(2~{S})-4-[[(2~{S},3~{S},4~{R},5~{R})-5-(6-aminopurin-9-yl)-3-[[(2~{R},3~{S},4~{R},5~{R})-5-(6-aminopurin-9-yl)-3,4-bis(oxidanyl)oxolan-2-yl]methoxy-oxidanyl-phosphoryl]oxy-4-oxidanyl-oxolan-2-yl]methylsulfanyl]-2-azanyl-butanoic acid | C24 H32 N11 O11 P S | 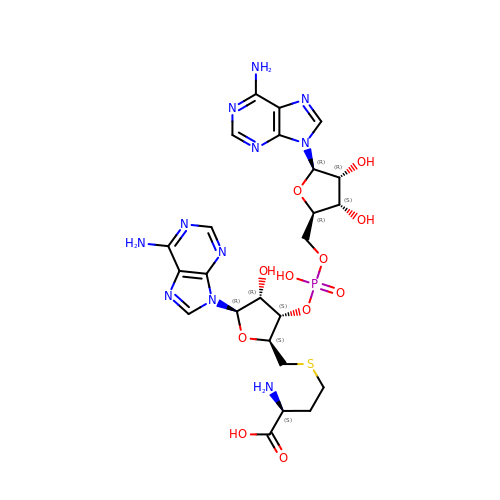QBCXMARFZQJLMA-XPJWLEQASA-N> MDRDTKLAFRLRGSHSRRTDDIDDDVIVFKTPNAVYREENSPIQSPVQPILSSPKLANSFEFPITTNNVNAQDRHEHGYQPLDAEDYPMIDSENKSLISESPQNVRNDEDLTT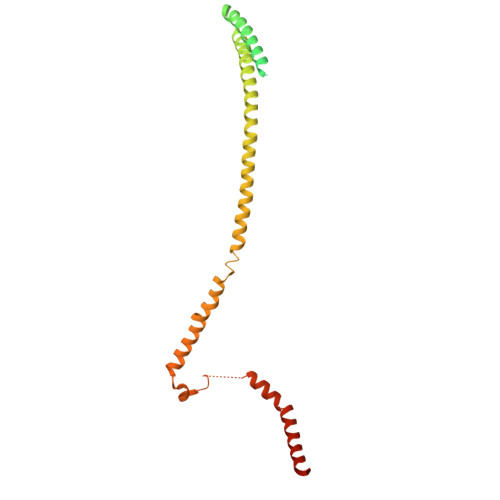RYNFDDIPIRQLSSSITSVTTIDVLSSLFINLFENDLIPQALKDFNKSDDDQFRKLLYKLDLRLFQTISDQMTRDLKDILDINVSNNELCYQLKQVLARKEDLNQQIISVRNEIQELKAGKDWHDLQNEQAKLNDKVKLNKRLNDLTSTLLGKYEGDRKIMSQDSEDDSIRDDSNILDIAHFVDLMDPYNGLLKKINKINENLSNELQPSLHHHHHH> SCSKCRKEMGQVEI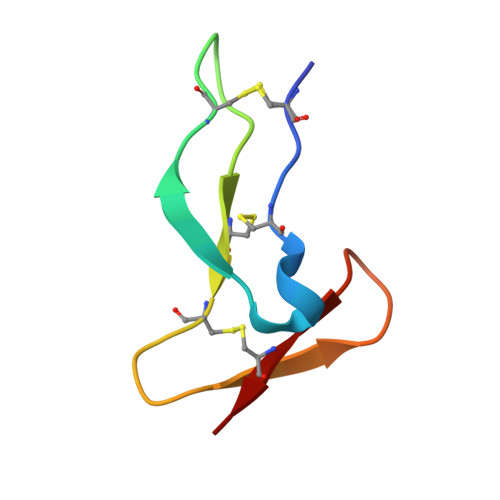SSCTVDRDTVCGCRKNQYRHYWSENLFQCFN>MPVFHTRTIESILEPVAQQISHLVIMHEEGEVDGKAIPDLTAPVAAVQAAVSNLVRVGKETVQTTEDQILKRDMPPAFIKVENACTKLVQAAQMLQSDPYSVPARDYLIDGSRGILSGTSDLLLTFDEAEVRKIIRVCKGILEYLTVAEVVETMEDLVTYTKNLGPGMTKMAKMIDERQQELTHQEHRVMLVNSMNTVKELLPVLISAMKIFVTTKNSKNQGIEEALKNRNFTVEKMSAEINEIIRVLQLTSWDEDAWASKDTEAMKRALASIDSKLNQAKGWLRDPSASPGDAGEQAIRQ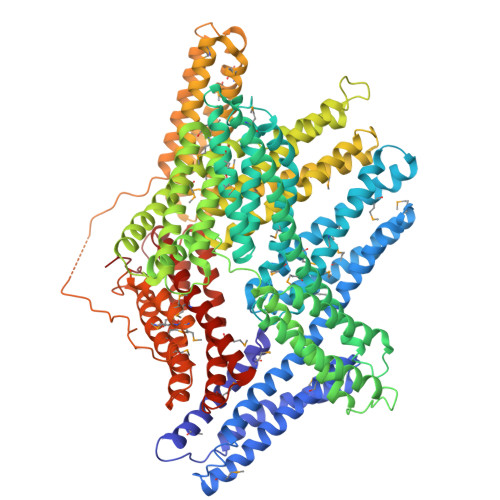ILDEAGKVGELCAGKERREILGTCKMLGQMTDQVADLRARGQGSSPVAMQKAQQVSQGLDVLTAKVENAARKLEAMTNSKQSIAKKIDAAQNWLADPNGGPEGEEQIRGALAEARKIAELCDDPKERDDILRSLGEISALTSKLADLRRQGKGDSPEARALAKQVATALQNLQTKTNRAVANSRPAKAAVHLEGKIEQAQRWIDNPTVDDRGVGQAAIRGLVAEGHRLANVMMGPYRQDLLAKCDRVDQLTAQLADLAARGEGESPQARALASQLQDSLKDLKARMQEAMTQEVSDVFSDTTTPIKLLAVAATAPPDAPNREEVFDERAANFENHSGKLGATAEKAAAVGTANKSTVEGIQASVKTARELTPQVVSAARILLRNPGNQAAYEHFETMKNQWIDNVEKMTGLVDEAIDTKSLLDASEEAIKKDLDKCKVAMANIQPQMLVAGATSIARRANRILLVAKREVENSEDPKFREAVKAASDELSKTISPMVMDAKAVAGNISDPGLQKSFLDSGYRILGAVAKVREAFQPQEPDFPPPPPDLEQLRLTDELAPPKPPLPEGEVPPPRPPPPEEKDEEFPEQKAGEVINQPMMMAARQLHDEARKWSSKGNDIIAAAKRMALLMAEMSRLVRGGSGTKRALIQCAKDIAKASDEVTRLAKEVAKQCTDKRIRTNLLQVCERIPTISTQLKILSTVKATMLGRTNISDEESEQATEMLVHNAQNLMQSVKETVREAEAASIKIRTDAGFTLRWVRKTPWYQ[2x]A pivotal component of the calcium (Ca2+) signaling toolbox in cells is the inositol 1,4,5-triphosphate (IP3) receptor (IP3R), which mediates Ca2+ release from the endoplasmic reticulum (ER), controlling cytoplasmic and organellar Ca2+ concentrations. IP3Rs are co-activated by IP3 and Ca2+, inhibited by Ca2+ at high concentrations, and potentiated by ATP. There are three IP3R subtypes (IP3R-1, -2, and -3) that share 60–70% sequence identity, form homo- or hetero-tetramers, exhibit different spatial expression profiles, and are involved in different signaling pathways. Each IP3R subunit is about 2700 amino acids in length and contains a transmembrane domain (TMD) and a large cytoplasmic region comprising two β-trefold domains (βTF1 and βTF2), three Armadillo repeat domains (ARM1, ARM2, and ARM3), a central linker domain (CLD), a juxtamembrane domain (JD), and a short C-terminal domain (CTD)6–10. Here we report cryo-electron microscopy (cryo-EM) structures of human type-3 IP3R obtained from a single dataset in multiple gating conformations: IP3-ATP bound pre-active states with closed channels, IP3-ATP-Ca2+ bound active state with an open channel, and IP3-ATP-Ca2+ bound inactive state with a closed channel.

The structure named “active” displays drastic conformational changes at the TMD, leading to pore opening. In addition to the well-resolved densities for IP3 and ATP, the active structure reveals substantial density, interpreted as Ca2+, at the ARM3-JD interface, referred to as the activatory Ca2+ binding site. Ca2+ is coordinated by E1882 and E1946 on the ARM3 and the main-chain carboxyl group of T2581 on the JD. When Ca2+ is bound, the JD rotates about 11° relative to the ARM3, resembling a clamshell closure, which leads to global conformational changes in the whole receptor, including the movement of the NTD closer to the membrane plane by 2 Å. In contrast to the limited rotation of the ARM3 (about 5°), the JD rotates about 14° around an axis roughly perpendicular to the membrane plane, leading to conformational changes at the TMD and resulting in pore opening in the active state. JD’s rotation upon Ca2+ binding pushes the pVSD’s cytoplasmic side away from the pore domain by about 7 Å and tilts the cytoplasmic side of the S6 (S6cyt) by 12°. Concurrently, the S4-5 linker and S5 helix move away from the S6 helix, thereby inducing a distortion of S6 around the constriction site and moving F2513 and I2517 away from the pore. As a result, the diameter of the water-accessible pore increases to 8 Å, large enough to permeate hydrated cations. The tilting of the S6cyt breaks the salt bridge between D2518 and R2524 of the neighboring subunits, moving D2518 towards the pore while pulling R2524 away, which creates an electronegative path on the cytoplasmic side of the pore.

>[4x]MSEMSSFLHIGDIVSLYAEGSVNGFISTLGLVDDRCVVEPAAGDLDNPPKKFRDCLFKVCPMNRYSAQKQYWKAKQTKQDKEKIADVVLLQKLQHAAQMEQKQNDTENKKVHGDVVKYGSVIQLLHMKSNKYLTVNKRLPALLEKNAMRVTLDATGNEGSWLFIQPFWKLRSNGDNVVVGDKVILNPVNAGQPLHASNYELSDNAGCKEVNSVNCNTSWKINLFMQFRDHLEEVLKGGDVVRLFHAEQEKFLTCDEYKGKLQVFLRTTLRQSATSATSSNALWEVEVVHHDPCRGGAGHWNGLYRFKHLATGNYLAAEENPSYKGDASDPKAAGMGAQGRTGRRNAGEKIKYCLVAVPHGNDIASLFELDPTTLQKTDSFVPRNSYVRLRHLCTNTWIQSTNVPIDIEEERPIRLMLGTCPTKEDKEAFAIVSVPVSEIRDLDFANDASSMLASAVEKLNEGFISQNDRRFVIQLLEDLVFFVSDVPNNGQNVLDIMVTKPNRERQKLMREQNILKQVFGILKAPFREKGGEGPLVRLEELSDQKNAPYQHMFRLCYRVLRHSQEDYRKNQEHIAKQFGMMQSQIGYDILAEDTITALLHNNRKLLEKHITKTEVETFVSLVRKNREPRFLDYLSDLCVSNHIAIPVTQELICKCVLDPKNSDILIRTELRPVKEMAQSHEYLSIEYSEEEVWLTWTDKNNEHHEKSVRQLAQEARAGNAHDENVLSYYRYQLKLFARMCLDRQYLAIDEISQQLGVDLIFLCMADEMLPFDLRASFCHLMLHVHVDRDPQELVTPVKFARLWTEIPTAITIKDYDSNLNASRDDKKNKFANTMEFVEDYLNNVVSEAVPFANEEKNKLTFEVVSLAHNLIYFGFYSFSELLRLTRTLLGIIDCVQGPPAMLQAYEDPGGKNVRRSIQGVGHMMSTMVLSRKQSVFSAPSLSAGASAAEPLDRSKFEENEDIVVMETKLKILEILQFILNVRLDYRISYLLSVFKKEFVEVFPMQDSGADGTAPAFDSTTANMNLDRIGEQAEAMFGVGKTSSMLEVDDEGGRMFLRVLIHLTMHDYAPLVSGALQLLFKHFSQRQEAMHTFKQVQLLISAQDVENYKVIKSELDRLRTMVEKSELWVDKKGSGKGEEVEAGAAKDKKERPTDEEGFLHPPGEKSSENYQIVKGILERLNKMCGVGEQMRKKQQRLLKNMDAHKVMLDLLQIPYDKGDAKMMEILRYTHQFLQKFCAGNPGNQALLHKHLHLFLTPGLLEAETMQHIFLNNYQLCSEISEPVLQHFVHLLATHGRHVQYLDFLHTVIKAEGKYVKKCQDMIMTELTNAGDDVVVFYNDKASLAHLLDMMKAARDGVEDHSPLMYHISLVDLLAACAEGKNVYTEIKCTSLLPLEDVVSVVTHEDCITEVKMAYVNFVNHCYVDTEVEMKEIYTSNHIWTLFENFTLDMARVCSKREKRVADPTLEKYVLSVVLDTINAFFSSPFSENSTSLQTHQTIVVQLLQSTTRLLECPWLQQQHKGSVEACIRTLAMVAKGRAILLPMDLDAHISSMLSSGASCAAAAQRNASSYKATTRAFPRVTPTANQWDYKNIIEKLQDIITALEERLKPLVQAELSVLVDVLHWPELLFLEGSEAYQRCESGGFLSKLIQHTKDLMESEEKLCIKVLRTLQQMLLKKTKYGDRGNQLRKMLLQNYLQNRKSTSRGDLPDPIGTGLDPDWSAIAATQCRLDKEGATKLVCDLITSTKNEKIFQESIGLAIHLLDGGNTEIQKSFHNLMMSDKKSERFFKVLHDRMKRAQQETKSTVAVNMNDLGSQPHEDREPVDPTTKGRVASFSIPGSSSRYSLGPSLRRGHEVSERVQSSEMGTSVLIMQPILRFLQLLCENHNRDLQNFLRCQNNKTNYNLVCETLQFLDIMCGSTTGGLGLLGLYINEDNVGLVIQTLETLTEYCQGPCHENQTCIVTHESNGIDIITALILNDISPLCKYRMDLVLQLKDNASKLLLALMESRHDSENAERILISLRPQELVDVIKKAYLQEEERENSEVSPREVGHNIYILALQLSRHNKQLQHLLKPVKRIQEEEAEGISSMLSLNNKQLSQMLKSSAPAQEEEEDPLAYYENHTSQIEIVRQDRSMEQIVFPVPGICQFLTEETKHRLFTTTEQDEQGSKVSDFFDQSSFLHNEMEWQRKLRSMPLIYWFSRRMTLWGSISFNLAVFINIIIAFFYPYMEGASTGVLDSPLISLLFWILICFSIAALFTKRYSIRPLIVALILRSIYYLGIGPTLNILGALNLTNKIVFVVSFVGNRGTFIRGYKAMVMDMEFLYHVGYILTSVLGLFAHELFYSILLFDLIYREETLFNVIKSVTRNGRSILLTALLALILVYLFSIVGFLFLKDDFILEVDRLPNNHSTASPLGMPHGAAAFVDTCSGDKMDCVSGLSVPEVLEEDRELDSTERACDTLLMCIVTVMNHGLRNGGGVGDILRKPSKDESLFPARVVYDLLFFFIVIIIVLNLIFGVIIDTFADLRSEKQKKEEILKTTCFICGLERDKFDNKTVSFEEHIKLEHNMWNYLYFIVLVRVKNKTDYTGPESYVAQMIKNKNLDWFPRMRAMSLVXXXXXXXXXXXXXXXXXXXXXX>[4x]GKIKIGINGFGRIGRLVARVALQSEDVELVAVNDPFITTDYMTYMFKYDTVHGQWKHSDIKIKDSKTLLLGEKPVTVFGIRNPDE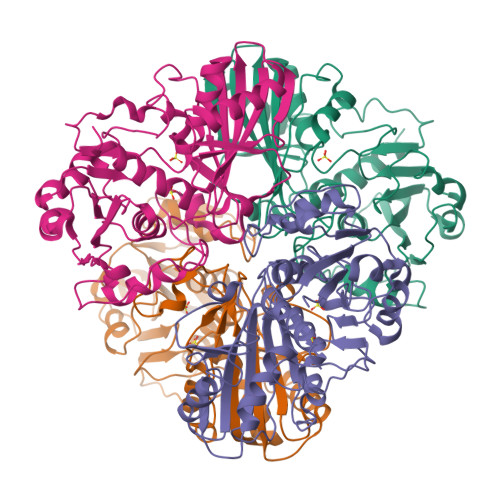IPWAEAGAEYVVESTGVFTDKEKAAAHLKGGAKKVVISAPSKDAPMFVCGVNEDKYTSDIDIVSNASCTTNCLAPLAKVIHDNFGIIEGLMTTVHAITATQKTVDGPSSKDWRGGRAASFNIIPSSTGAAKAVGKVLPDLNGKLTGMSFRVPTVDVSVVDLTVRIEKAASYDAIKSAIKSASEGKLKGIIGYVEEDLVSTDFVGDSRSSIFDAKAGIALNDNFVKLVAWYDNEWGYSNRVIDLIRHMAKTQ> QLPPGKPEIFKCRSPNKETFTCWWRPGTDGGLPTNYSLTYHREGETLMHECPDYITGGPNSCHFGKQYTSMWRTYIMMVNATNQMGSSFSDELYVDVTY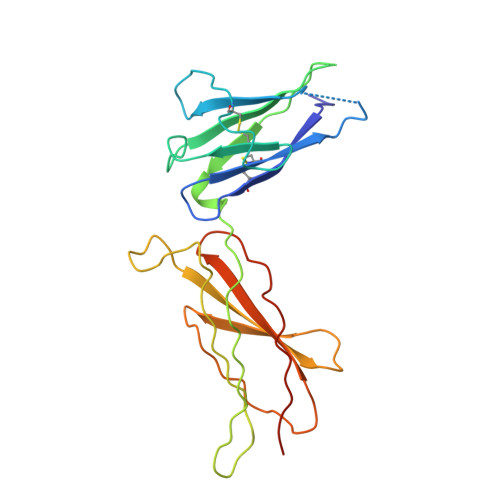IVQPDPPLELAVEVKQPEDRKPYLWIKWSPPTLIDLKTGWFTLLYEIRLKPEKAAEWEIHFAGQQTEFKILSLHPGQKYLVQVRCKPDHGYWSAWSPATFIQIPSDFTMNDT> GSHMASMKKKGSVVIVG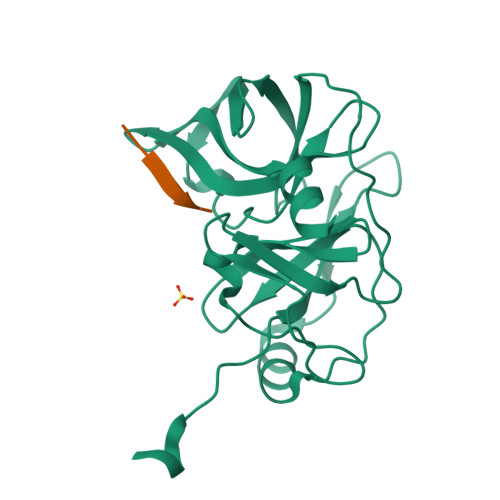RINLSGDTAYAQQTRGEEGCQETSQTGRDKNQVEGEVQIVSTATQTFLATSINGVLWTVYHGAGTRTIASPKGPVTQMYTNVDKDLVGWQAPQGSRSLTPCTCGSSDLYLVTRHADVIPVRRRGDSRGSLLSPRPISYLKGSAGGPLLCPAGHAVGIFRAAVSTRGVAKAVDFIPVESLETTMRSP;> PPPPPPPPSSTPC>[4x]MSQHNEKNPHQHQSPLHDSSEAKPGMDSLAPEDGSHSPAAEPTPPGAQPTAPGSLKAPDTRNEKLNSLEDVRKGSENYALTTNQGVRIADDQNSLRAGDRGPTLLEDFILREKITHFDHERIPERIVHARGSAAHGYFQPYKSLSDITKADFLSDPNKITPVFVRFSTVQGGAGSADTVRDIRGFATKFYTEEGIFDLVGNNTPIFFIQDAHKFPDFVHAVKPEPHWAIPQGQSAHDTFWDYVSLQPETLHNVMWAMSDRGIPR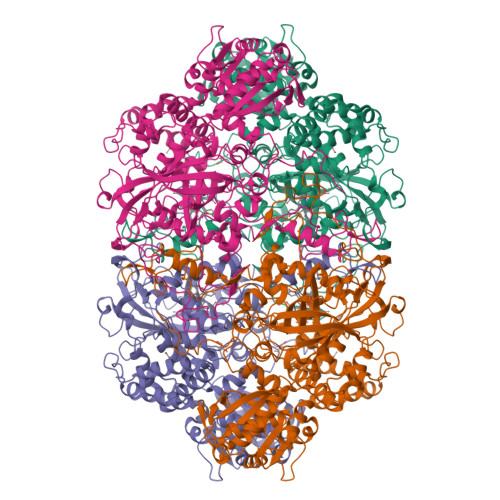SYRTMEGFGIHTFRLINAEGKATFVRFHWKPLAGKASLVWDEAQKLTGRDPDFHRRELWEAIEAGDFPEYELGFQLIPEEDEFKFDFDLLDPTKLIPEELVPVQRVGNMVLNRNPDNFFAENEQAAFHPGHIVPGLDFTNDPLLQGRLFSYTDTQISRLGGPNFHEIPINRPTCPYHNFQRDGMHRMGIDTNPANYEPNSINDNWPRETPPGPKRGGFESYQERVEGNKVRERSPSFGEYYSHPRLFWLSQTPFEQSHIVDGFSFELSKVVRPYIRERVVDQLAHIDLTLAQAVAKNLGIELTDDQLNITPPPDVNGLKKDPSLSLYAIPDGDVKGRVVAILLNDEVRSADLLAILKALKAKGVHAKLLYSRMGEVTADDGTVLPIAATFAGAPSLTVDAVIVPCGNIADIADNGDANYYLMEAYKHLKPIALAGDARKFKATIKIADQGEEGIVEADSADGSFMDELLTLMAAHRVWSRIPKIDKIPA Many folds, spanning all levels of complexity (fibrous, solenoid, toroid, and globular), clearly originated in this way. β-Propellers offer an attractive model system to study this process. They are toroids formed by sequential supersecondary structure units of typically 40–50 residues, each consisting of four anti-parallel β-strands. The units are arranged radially, with their strands perpendicular to the plane of the toroid, and have a right-handed twist, hence the name ‘propeller’ for the fold and ‘blades’ for the repetitive units. Since none of our single-bladed PkwA constructs were folded, we turned our attention to another highly symmetric β-propeller of the WD40 family, found in the C-terminal part of Npun_R6612 from the multicellular cyanobacterium Nostoc punctiforme PCC 73102 and referred to henceforth as WRAP (WD40-family Recently Amplified Propeller; ACC84870.1). WRAP, which we identified during a systematic bioinformatic survey of β-propellers, was particularly interesting in that its 14 blades are practically identical, having acquired only 10 point mutations over 563 residues (6 of these being Trp → Arg mutations at the same position of blades 1, 3, 6, 10, 12, and 13), as a result of 13 non-synonymous substitutions at the DNA level.

The 5-bladed fragment, however, did not form a 10-bladed propeller, even though it was dimeric, as observed in solution. Rather, the dimer adopted an unusual, asymmetric structure, hitherto unseen in natural proteins, in which one monomer formed the expected 5 blades of an incomplete propeller, while the other monomer formed only four blades and converted part of the N-terminal fifth blade to a helix, leaving the rest of this blade unstructured. The blades in one monomer were antiparallel to the blades in the other, as opposed to natural propellers, where the blades are always parallel. Thus, while the fold is clearly built of blades, it is not a propeller. As the stretch of sequence preceding the helix was not resolved in the structure, we analyzed the intactness of the crystallized protein and found that it had undergone partial trimming during crystallization. Instead, one monomer changes orientation, improving the geometry at one of the two interfaces, and compensates for the accumulated tension at the other interface by conversion of its N-terminal blade to a helix, thus also reducing to nine the number of blades that have to be accommodated in the structure. The change in its genetic information is not large, going from 2, 3, 4, or seven repeat units to 5, but it is certainly discontinuous and leads to the sudden emergence of a new form, which – as a stable, efficiently folded protein – is available for further evolution.

>[4x]GAMGSSSVWGVAFSPDGQTIASASDDKTVKLWNRNGQLLQTLTGHSSSVWGVAFSPDGQTIASASDDKTVKLWNRNGQLLQTLTGHSSSVWGVAFSPDGQTIASASDDKTVKLWNRNGQLLQTLTGHSSSVWGVAFSPDGQTIASASDDKTVKLWNRNGQLLQTLTGHSSSVWGVAFSPDGQTIASASDDKTVKLWNRNGQLLQTLTGH> GANSLSVHQLAAQGEMLYLATRIEQENVINHTDEEGFTPLMWAAAHGQIAVVEFLLQNGADPQLLGKGRESALSLACSKGYTDIVKMLLDCGVDVNEYDWNGGTPLLYAVHGNHVKCVKMLLESGADPTIETDSGYNSMDLAVALGYRSVQQV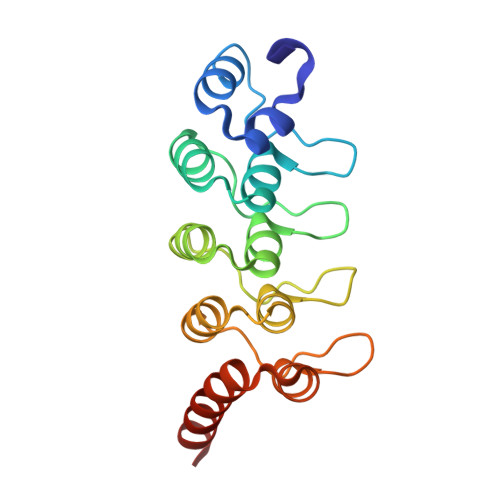IESHLLKLLQNIKE> VFHKIRNEDLIFNESLGQGTFTKIFKGVRREVGDYGQLHETEVLLKVLDKAHRNYSESFFEAASMMSKLSHKHLVLNYGVCVCGDENILVQEFVKFGSLDTYLKKNKNCINILWKLEVAKQLAAAMHFLEENTLIHGNVCAKNILLIREEDRKTGNPPFIKLSDPGISITVLPKDILQERIPWVPPECIENPKNLNLATDKWSFGTTLWEICSGGDKPLSALDSQRKL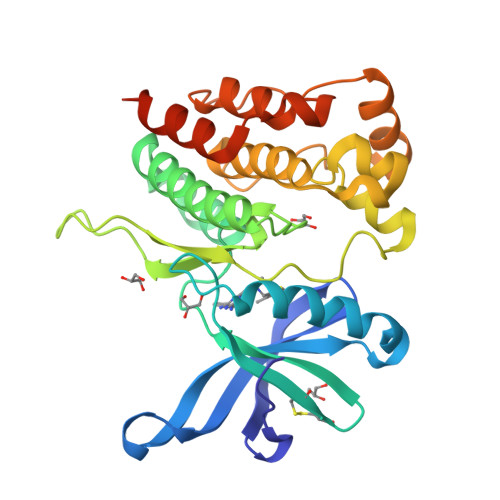QFYEDRHQLPAPKAAELANLINNCMDYEPDHRPSFRAIIRDLNSLFTPDLVPRGSHHHHHH>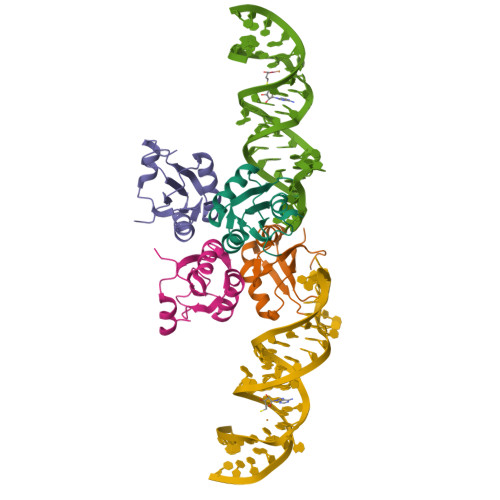[4x]MAVPETRPNHTIYINNLNEKIKKDELKKSLYAIFSQFGQILDILVSRSLKMRGQAFVIFKEVSSATNALRSMQGFPFYDKPMRIQYAKTDSDIIAKMKGTFV> DSWKDGC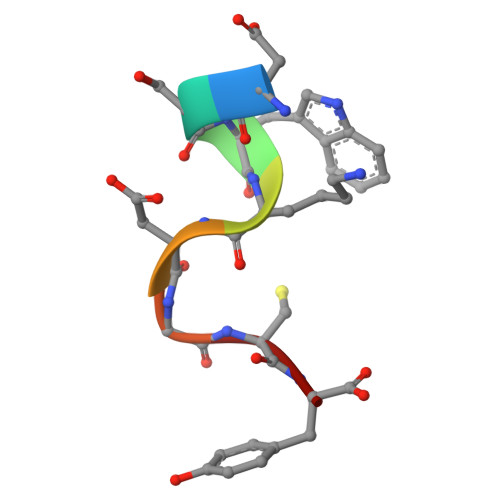Y1-[(3~{R})-3-azanylpiperidin-1-yl]-4,4,4-tris(fluoranyl)butan-1-one | C9 H15 F3 N2 O | 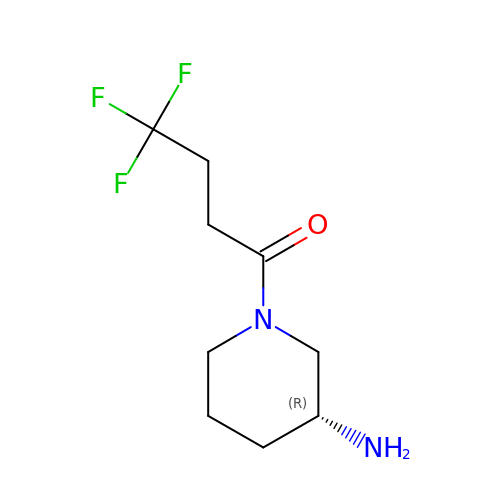GPYQCFFYXYYNET-SSDOTTSWSA-N> DQELGKQSRRSQDIIKSLGFLSSDQKDILVKSISSSKDSQLILKFVTQATQLNNAESTKAKQMAQNDVALIKNISPEVLEEYKEKIQRASTKSQ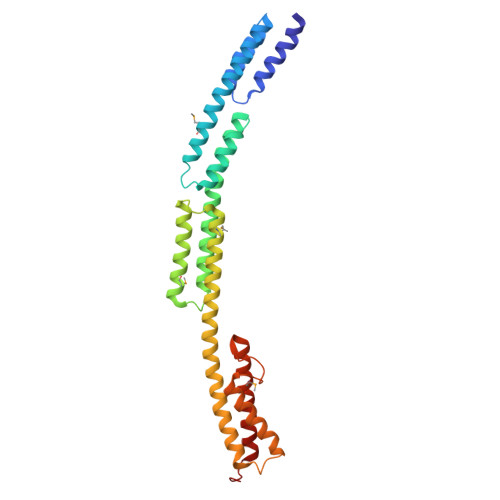VDEFVAEAKKVVNSNKETLVNQANGKKQEIAKLENLSNDEMLRYNTAIDNVVKQYNEGKLNITAAMNALNSIKQAAQEVAQKNLQKQYAKKIERISSKGLALSKKAKEIYEKHKSILPTPGYYADSVGTYLNRFRDKQTFGNRSVWTGQSGLDEAKKMLDEVKKLLKELQDLTRGTKED> GPGSTQQDVCKWLKKHCPNQYQLYSESFKQHDITGRALLRLTDKKLERMGIAQENQRQHILQQVLQLKVREEVRNLQLLTQASVECSPGS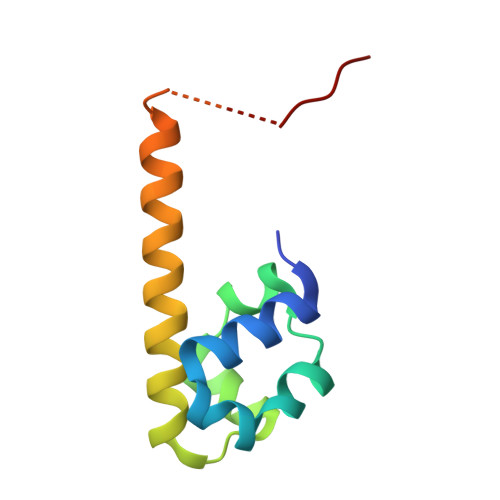GSENLYFQ>[4x]MMENIMKKRLLSTSISTLLLGLSVMPAFADEDVTAWRLFIADHDKPVVNVIDALDGDKLATFNVKGPANLSRSESGATIFAIQGSAGVVSTIASGIAFHDHGDHADIDIDAPKLLPLELTGKKPGHFVERQGKIAQWFDGEDSAQILGESAVLKGQKNITKVNVVAPHHGVAVPYDNYAVVSIPNPDDASKRPVGARVVDLQGKKVGDDALCPGLHGSAGSGDTFALSCETGLLLITQKNAAPVIRHLPYAKTLPEGSTSTLIGGKGMQYFIGNYGPDRIILVDPTESDSFRLIQLPTRRVHFVVDPVRAKFAYVFTEDGKLNQIDVLKGEISQSVRVTDPYSMDGHWNDPRPRIAVADNKIYVTDPLKSKIIVLDATSFKKTSEISVEGQPFNIVAVGGSGKVHGEHHDHEAHHHDDHAH

We have recently identified a periplasmic protein AztD in Paracoccus denitrificans, which is able to transfer zinc to the cluster A-I SBP AztC23. Here, we describe crystal structures of AztD homologs from P. denitrificans (PdAztD) and Citrobacter koseri (CkAztD), a pathogen of the carbapenem-resistant Enterobacteriacea group. In each case, the protein adopts a beta-propeller fold composed of continuous antiparallel beta sheets forming 8, 3-, and 4-stranded blades and containing a disulfide bond between highly conserved Cys214 and Cys231 (P. denitrificans numbering). Two high-affinity zinc-binding sites are identified, only one of which is competent for transfer to AztC.

Poorly occupied sites also exhibited weak 2Fo–Fc density for ligand residues, indicative of disorder when zinc is absent. Indeed, although the crystal structures of apo and holo CkAztD are very similar overall (RMSD = 0.22–0.44 Å), residues 99–104, including zinc ligands His101 and His104, could not be modeled in three of four chains of the apo structure. In the chain where these residues could be modeled, they were displaced from their positions in the holo structure. The C terminus including His405 was disordered in all chains. In contrast, very little structural perturbation occurs for ligands to site 1 when zinc is absent.> MTITIKPPKGNGAPVPVETTLVKKVNADGVLTFDILENKYTYEVINAIGKRWIVSHVEGENDKKEYVITVIDRKSEGDRQLVECTAREIPIDKLMIDRIYVNVTGSFTVERYFNIVFQGTGMLFEVEGKVKSSKFENGGEGDTRLEMFKKGLEHFGLEYKITYDKKKDRYKFVLTPFANQKASYFISDEVNANAIKLEEDASDFATFIRGYGNYSGEETFEHAGLVMEARSALAEIYGDIHAEPFKDGKVTDQETMDKELQSRLKKSLKQSLSLDFLVLRESYPEADPQPG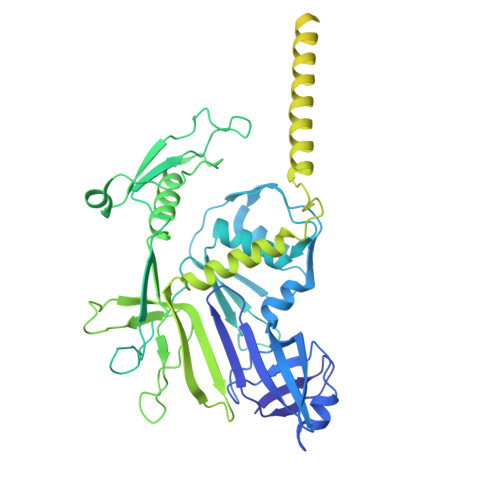DIVQIKSTKLGLNDLVRIVQVKTIRGINNVIVKQDVTLGEFNREQRYMKKVNTAANYVSGLNDVNLSNPSKAAENLKSKVASIAKSTLDLMSRTDLIEDKQQKVSSKTVTTSDGTIVHDFIDKSNIKDVKTIGTIGDSVARGSHAKTNFTEMLGKKLKAKTTNLARGGATMATVPIGKEAVENSIYRQAEQIRGDLIILQGTDDDWLHGYWAGVPIGTDKTDTKTFYGAFCSAIEVIRKNNPASKILVMTATRQCPMSGTMIRRKDTDKNKLGLTLEDYVNAQILACSELDVPVYDAYHTDYFKPYNPAFRKSSMPDGLHPNERGHEVIMYELIKNYYQFYG> MSSIKKISFVGIFSALATLVMFLEFPIFPQASFLKYDPSEIPALIVSFLL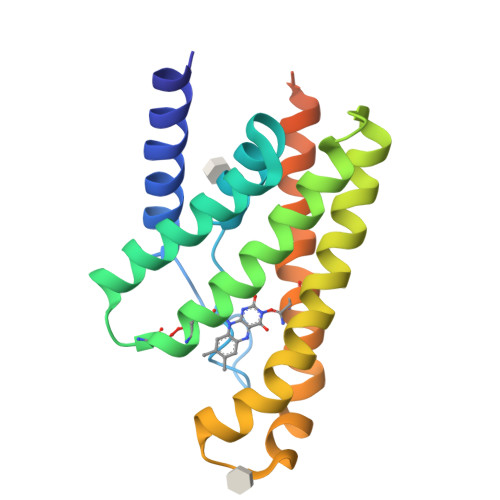GPGVGMFVVLVKDILFFLMKSGDPVGIAMNAVLGMSFVGIAGLIYHRNKSRATAIKGMIVATLFATAFALGLNALIVPLYFEAPFELYLKFFPFILAFNLVKFGIDSVVTFFVYKKVSSILKLETVEGRSNNGSNSLVPR> GDLKKVLNFHFS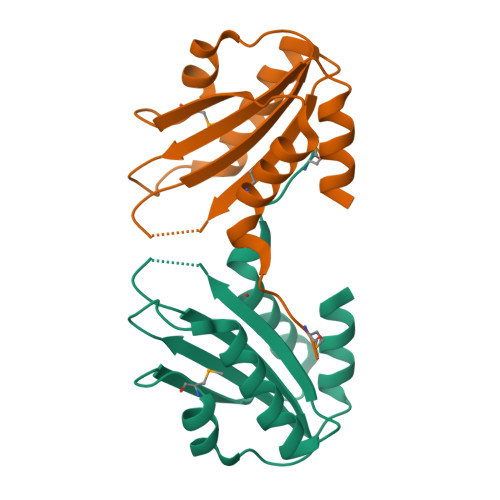YIYTYFITITTNYKYGDTEKIFRKFRSYIYNHDKNSHVFSIKETTKNSNGLHYHILVFTNKKLDYSRVHKHMPSHSDIRIELVPKSISDIKNVYKYMLKTKKDIKMS>[2x]GPHMADLMSSSPLSKKRRVSGPDPKPGSNCSPAQSVLSEVPSVPTNGMAKNGSEADIDEGLYSRQLYVLGHEAMKRLQTSSVLVSGLR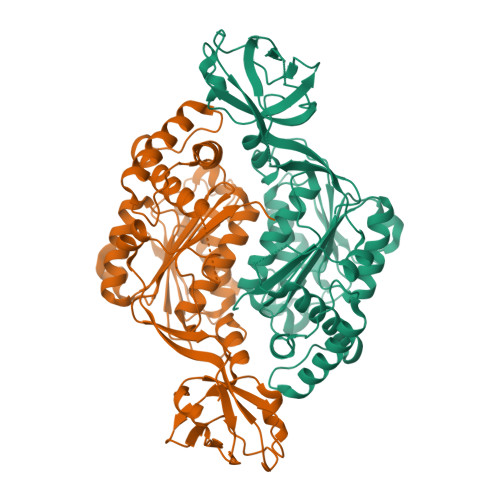GLGVEIAKNIILGGVKAVTLHDQGTAQWADLSSQFYLREEDIGKNRAEVSQPRLAELNSYVPVTAYTGPLVEDFLSGFQVVVLTNTPLEDQLRVGEFCHNRGIKLVVADTRGLFGQLFCDFGEEMILTDSNGEQPLSAMVSMVTKDNPGVVTCLDEARHGFESGDFVSFSEVQGMVELNGNQPMEIKVLGPYTFSICDTSNFSDYIRGGIVSQVKVPKKISFKSLVASLAEPDFVVTDFAKFSRPAQLHIGFQALHQFCAQHGRPPRPRNDEDAAELVALAQAVNARALPAVQQNNLDEDLIRKLAYVAAGDLAPINAFIGGLAAQEVMKACSGKFMPIMQWLYFDALECLPEDKEVL> MKA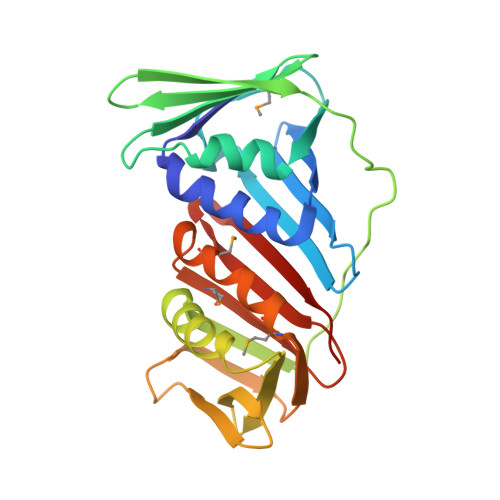KVIDAVSFSYILRTVGDFLSEANFIVTKEGIRVSGIDPSRVVFLDIFLPSSYFEGFEVSQEKEIIGFKLEDVNDILKRVLKDDTLILSSNESKLTLTFDGEFTRSFELPLIQVESTQPPSVNLEFPFKAQLLTITFADIIDELSDLGEVLNIHSKENKLYFEVIGDLSTAKVELSTDNGTLLEASGADVSSSYGMEYVANTTKMRRASDSMELYFGSQIPLKLRFKLPQEGYGDFYIAPRAD>ADPQKLDDVDPLVTTNFGKIRGIKKELNNEILGPVIQFLGVPYAAPPTGEHRFQPPEPPSPWSDIRNATQFAPVCPQNIIDGRLPEVMLPVWFTNNLDVVSSYVQDQSEDCLYLNIYVPTEDDIRDSGGPKPVMVYIHGGSYMEGTGNLYDGSVLASYGNVIVITVNYRLGVLGFLSTGDQAAKGNYGLLDLIQALRWTSENIGFFGGDPLRITVFGSGAGGSCVNLLTLSHYSEKGLFQRAIAQSGTALSSWAVSFQPAKYARILATKVGCNVSDTVELVECLQKKPYKELVDQDVQPARYHIAFGPVIDGDVIPDDPQILMEQGEFLNYDIMLGVNQGEGLKFVENIVDSDDGVSASDFDFAVSNFVDNLYGYPEGKDVLRETIKFMYTDWADRHNPETRRKTLLALFTDHQWVAPAVATADLHSNFGSPTYFYAFYHHCQTDQVPAWADAAHGDEVPYVLGIPMIGPTELFPCNFSKNDVMLSAVVMTYWTNFAKTGDPNQPVPQDTKFIHTKPNRFEEVAWTRYSQKDQLYLHIGLKPRVKEHYRANKVNLWLELVPHLHNLNDHHHHHH[4x];>GSPGISGGGGGILEASSLGAHHIHHFHGSSKHHSVPIAIYRSPASLRGGHAGTTYIFSKGGGQITYKWPPNDRPSTRADRLAIGFSTVQKEAVLVRVDSSSGLGDYLELHIHQGKIGVKFNVGTDDIAIEESNAIINDGKYHVVRFTRSGGNATLQVDSWPVIERYPAGRQLTIFNSQATIIIGGKEQGQPFQGQLSGLYYNGLKVLNMAAENDANIAIVGN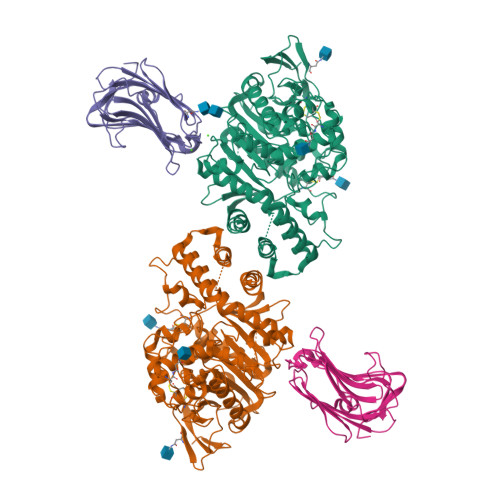VRLVGEVPSSMTTESHHHHHH[4x]> GTSQPVLRGDGARPSWLASALACVLIFTIVVDILGNLLVILSVYRNKKLRNAGNIFVVSLAVANLVVAIYPYPLVLMSIFNNGWNFGYLHCQVSAFLMGLSVIGSIWNITGIAIDRYLYICHSLKYDKLYSSKNSLCYVLLIWLLTLAAVLPNLRAGTLQYDPRIYSCTFAQSVSSAYTIAVVVFHFLVPMIIVIFCYLRIWILVLQVRGIDCSFWNESYLTGSRDERKKSLLSKFGMDEGVTFMFIGRFDRGQKGVDVLLKAIEILSSKKEFQEMRFIIIGKGDPELEGWARSLEEK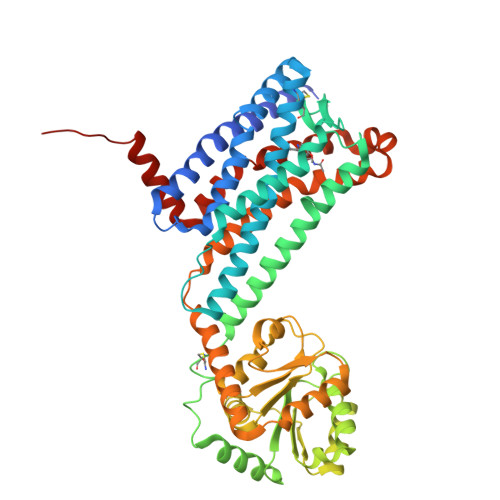HGNVKVITEMLSREFVRELYGSVDFVIIPSYFEPFGLVALEAMCLGAIPIASAVGGLRDIITNETGILVKAGDPGELANAILKALELSRSDLSKFRENCKKRAMSFSKLKPQDFRNFVTMFVVFVLFAICFAPLNFIGLAVASDPASMVPRIPEWLFVASYYMAYFNSCLNPIIYGLLDQNFRKEYRRIIVSLCTARVFFVDSSN> APTMTEFVGTAGGDTVGLVIANVDSLLHKHLGLDNTCRSIGIISARVGAPAQMMAADEAVKGTNTEVATIELPRDTKGGAGHGIFIVLKAADVSDARRAVEIALKQTDKYLGNVYLCDAGHLEVQYTARASLIFEKAFGAPSGQAFGIMHAAPAGVGMIVADTALKTADVKLITYGSPTNGVLSYTNEILITISGDSGAVLQSLTAARKAGLSIL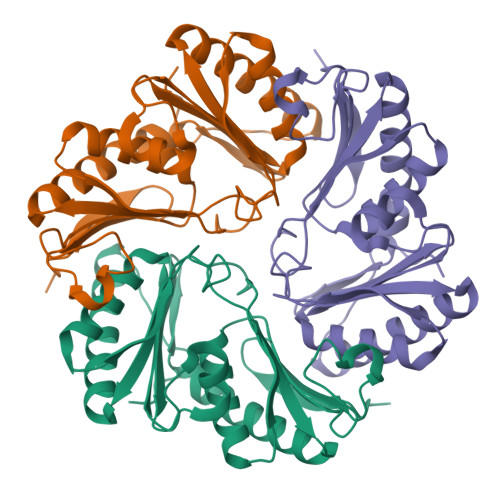RSMGQDPVSMSKPTF>[2x]GVYRVCVSTGASIYAGSKNKVELWLVGQHGEVELGSCLRPTRNKEEEFKVNVSKYLGSLLFVRLRKKHFLKEDAWFCNWISVQALGAA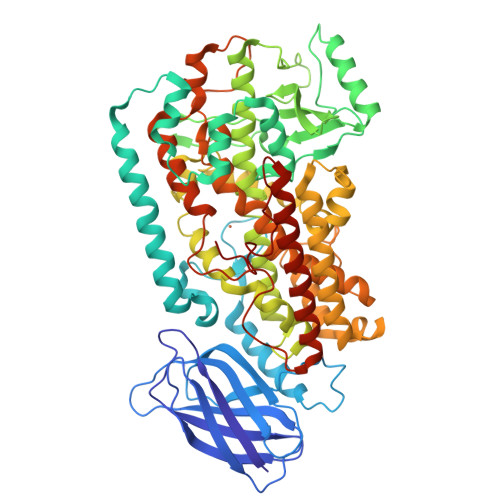EDKYWFPCYRWVVGDGVQSLPVGTGCTTVGDPQGLFQKHREQELEERRKLYQWGSWKEGLILNVAGSKLTDLPVDERFLEDKKIDFEASLAWGLAELALKNSLNILAPWKTLDDFNRIFWCGRSKLARRVRDSWQEDSLFGYQFLNGANPMLLRRSVQLPARLVFPPGMEELQAQLEKELKAGTLFEADFALLDNIKANVILYCQQYLAAPLVMLKLQPDGKLMPMVIQLHLPKIGSSPPPLFLPTDPPMVWLLAKCWVRSSDFQVHELNSHLLRGHLMAEVFTVATMRCLPSIHPVFKLIVPHLRYTLEINVRARNGLVSDFGIFDQIMSTGGGGHVQLLQQAGAFLTYRSFCPPDDLADRGLLGVESSFYAQDALRLWEIISRYVQGIMGLYYKTDEAVRDDLELQSWCREITEIGLQGAQKQGFPTSLQSVAQACHFVTMCIFTCTGQHSSIHLGQLDWFTWVPNAPCTMRLPPPTTKDATLETVMATLPNLHQSSLQMSIVWQLGRDQPIMVPLGQHQEEYFSGPEPRAVLEKFREELAIMDKEIEVRNEKLDIPYEYLRPSIVENSVAI>MPEGPELHLASQFVNEACRALVFGGCVEKSSVSRNPEVPFESSAYRISASARGKELRLILSPLPGAQPQQEPLALVFRFGMSGSFQLVPREELPRHAHLRFYTAPPGPRLALCFVDIRRFGRWDLGGKWQPGRGPCVLQEYQQFRENVLRNLADKAFDRPICEALLDQRFFNGIGNYLRAEILYRLKIPPFEKARSVLEALQQHRPSPELTLSQKIRTKLQNPDLLELCHSVPKEVVQLGGRGRGSESGEEDFAAFRAWLRCYGMPGMSSLQDRHGRTIWFQGDPGPLAPKGRKS[3x]

Human endonuclease VIII-like 1 (hNEIL1) is a bifunctional DNA glycosylase of the Fpg/Nei family, which catalyzes the removal of damaged bases and subsequent incision of the newly generated abasic sites. Unlike traditional enzymes which are commonly referred to as highly specific biocatalysts, one special feature for hNEIL1 is its unique capability to recognize a wide range of substrates, including formamidopyrimidines, hydantoin lesions, oxidized, and dihydro-modified pyrimidine bases, derived from all four canonical bases. Here, by integrating structural, computational, and biochemical investigations, we show that hNEIL1 uses a triage mechanism to achieve broad specificity and reduce futile repair of normal bases. This mechanism involves two mutually competing interaction states: an activated state that commits catalysis and BER, and a quarantine state that temporarily separates and prevents the flipped base from catalysis via auto-inhibition.

We synthesized a 2′-fluoro-substituted stable mimic of DHU (FDHU), which allows binding but not catalysis by hNEIL1. As a further test of the proposed mechanism, we also sought to “rescue” the activated state by mutating the lesion-recognition loop. Because a nearby positively charged amino acid side chain is important for catalysis, we attempted to introduce a charged residue in close proximity to the flipped base. Considering that Y244 is able to closely contact the base in the quarantine state, we envisioned that replacing Y244 with a positively charged residue might re-establish an active-state-like interaction between the mutated residue 244 and the flipped base, thus possibly rescuing the catalysis activity. To our delight, introduction of Y244R to hNEIL1(R242A) or hNEIL1(R242H) mutant resulted in both mutants to restore their glycosylase activity; in fact, we even found comparable or higher activity for hNEIL1(R242A, Y244R) and hNEIL1(R242H, Y244R) than the wild-type hNEIL1 for DHU and Tg. We further solved the crystal structure of hNEIL1(Y244R) bound to FDHU, and found that although the loop remains at the 244-in conformation, Arg244 forms a key hydrogen bond to the flipped base, recapitulating the key interaction in the activated state rather than the quarantine state. For instance, based on our mechanistic understanding, we rationally introduced an Arginine mutation to the 244 position of the catalytically incompetent hNEIL1(R242H) and hNEIL1(R242A) mutants, thereby creating new gain-of-function mutants.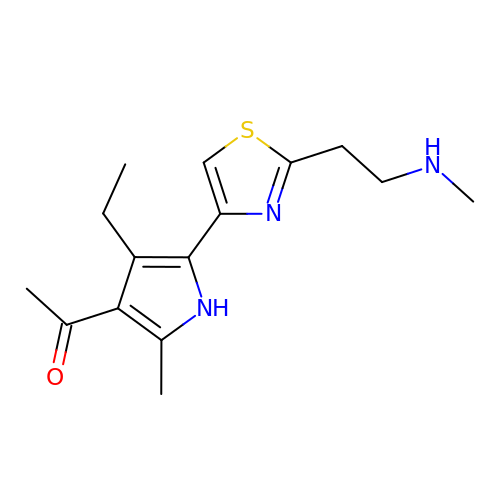1-[4-ethyl-2-methyl-5-[2-[2-(methylamino)ethyl]-1,3-thiazol-4-yl]-1~{H}-pyrrol-3-yl]ethanone | C15 H21 N3 O S | UTWAWNDFTMJUGN-UHFFFAOYSA-N>TKIPRGNGPYSVGCTDLMFDHTNKGTFLRLYYPSQDNDRLDTLWIPNKEYFWGLSKFLGTHWLMGNILRLLFGSMTTPANWNSPLRPGEKYPLVVFSHGLGAFRTLYSAIGIDLASHGFIVAAVEHRDRSASATYYFKDQSAAEIGDKSWLYLRTLKQEEETHIRNEQVRQRAKECSQALSLILDIDHGKPVKNALDLKFDMEQLKDSIDREKIAVIGHSFGGATVIQTLSEDQRFRCGIALDAWMFPLGDEVYSRIPQPLFFINSEYFQYPANIIKMKKCYSPDKERKMITIRGSVHQNFADFTFATGKIIGHMLKLKGDIDSNVAIDLSNKASLAFLQKHLGLHKDFDQWDCLIEGDDEN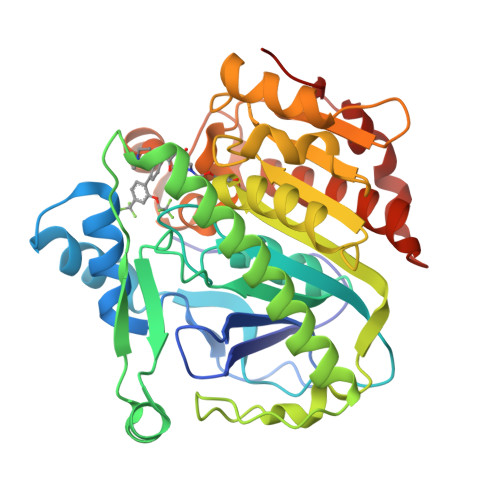LIPGTNI[2x]> SEDSRPAAHFHLSSRRRHQGSMGYHGDMYIGNDNERNSYQGHFQTRDGVLTVTNTGLYYVYAQICYNNSHDQNGFIVFQGDTPFLQCLNTVPTNMPHKVHTCHTSGLIHLERNERIHLKDIHNDRNAVLREGNNRSYFGI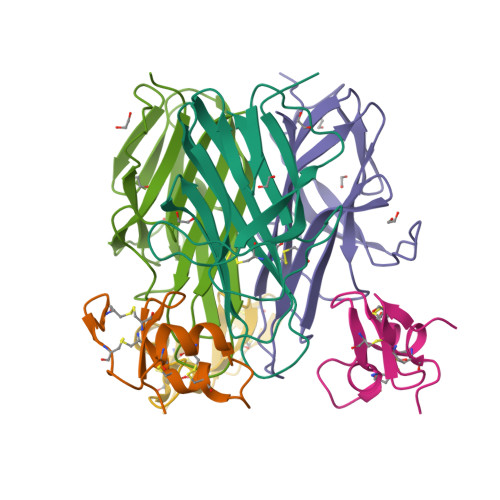FKV;> GESRDCHGTICHPVNEFCYVATERCHPCIEVCNNQTHNYDAFLCAKECSAYK>[2x]NENLS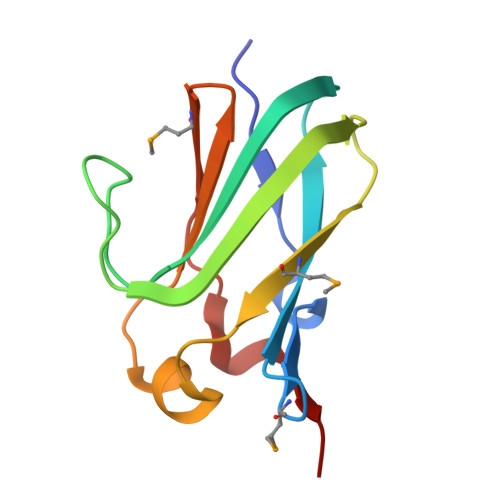FTVKTDRIVYDMTQQVITIPVKPNKSVNASDVHAVLTYGWDGNGSSEKVIGEVYLKDVQWTAGIEYTIMISAELSIDEIKSKDKVDLIVFYDGQMTITENLKPSSWTVVGP>MNKLTIIVTYYNAEEYITGCLESIKQQRTQDFNLIIVNDGSTDQSKKLMDEAIKDYDKNIRFIDLDENSGHAHARNIALEEVETPYFMFLDADDELASYAITFYLEKFNNTDGLIAPIHSFTTQRPQFVDLDRVRVEYFNAKENINSFLRKQSACNIIFRTAIVRAHHIRFNENLNTYVDWSFVLEYMKYVNKFVRIFNFPFYFRGEVYDPFETLTLSEQNFDILFKDYVNSFYDAIKRATNPKVREFIVTKMGNKIANEFEPTRYDINERYQTHKDTLVELSKFLHVHLVKNQKLINKIETILLMNNETDKAFKVNQFRKTLRHVKNIVLRRKNKERSLYDLTDKEDNVKPKTIVFESFGGKNYSDSPKYIYEYMQKYYPNYRYIWSFKNPDKNVVPGSAEKVKRNSAEYYQAYSEASHWVSNARTPLYLNKKENQTYIQTWHGTPLKRLANDMKVVRMPGTTTPKYKRNFNRETSRWDYLISPNRYSTEIFRSAFWMDEERILEIGYPRNDVLVNRANDQEYLDEIRTHLNLPSDKKVIMYAPTWRDDEFVSKGKYLFELKIDLDNLYKELGDDYVILLRMAYLISNALDLSGYENFAIDVSNYNDVSELFLISDCLITDYSSVMFDYGILKRPQFFFAYDIDKYDKGLR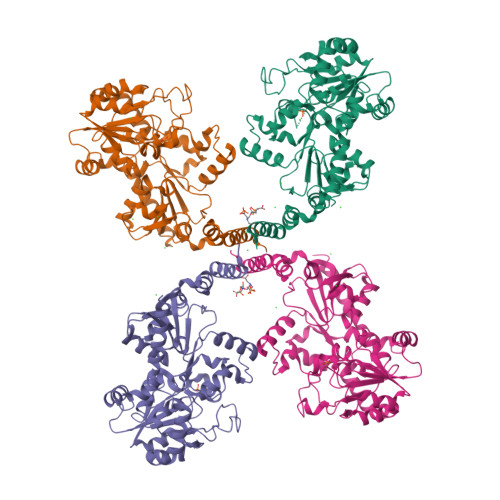GFYMNYMEDLPGPIYTEPYGLAKELKNLDKVQQQYQEKIDAFYDRFCSVDNGKASQYIGDLIHKDIKEQLEHHHHHH[4x]>[4x]MSNAEKALGVALIGTGFMGKCHAMAWRNVATAFGGLPPRLEVLADMPADKAHSLASSFGFARGTADWREAVSDPAVDVVSITTPNGLHREMAEAALA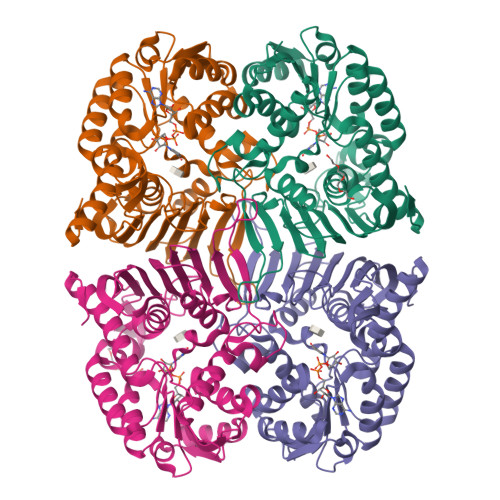AGKHVWLEKPMALSVEDAQAMEAAARASDRRTIIGYNYTRSPAFRAAVDLIAEGAIGRPIHFRGMYDEDYMADPDLPWSWALTRKDGGLGALGDLGCHLVSVMVSLMGPVARVYAQADTVITDRPHQGGTARVENEDQAQALIRFASGTSGEFSCSRVARGYRCRLAWEVQGTEGTLRFDQERMNELWLYQPGRPEIDGFRRILTGPAQPGFAAFCPGGGHNFGFNEQKVVEAEMLRQAIAGRGKAWPDFTDGLTIERVIHGMATSAQTGQPVNFLEHHHHHH> MRRHYRDLIRNTPMPDTPQDIADLRALLDEDEAEMSVVFSDPS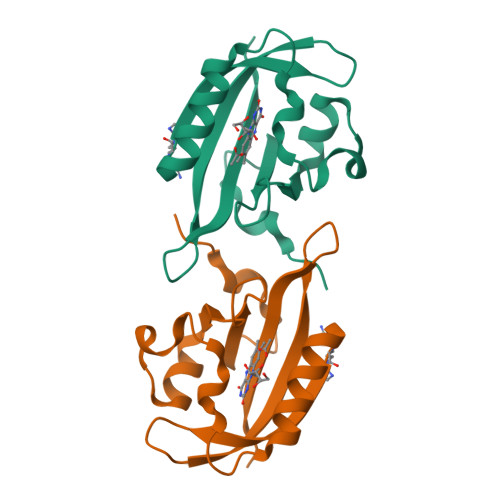QPDNPMIYVSDAFLVQTGYTLEEVLGRNCRFLQGPDTNPHAVEAIRQGLKAETRFTIDILNYRKDGSAFVNRLRIRPIYDPEGNLMFFAGAQNPVLEHHHHHH> MGDSILSQAEIDA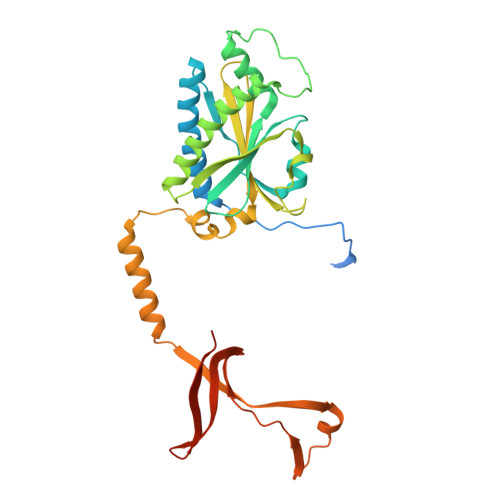LLNGDSDTKDEPTPGIASDSDIRPYDPNTQRRVVRERLQALEIINERFARQFRMGLFNLLRRSPDITVGAIRIQPYHEFARNLPVPTNLNLIHLKPLRGTGLVVFSPSLVFIAVDNLFGGDGRFPTKVEGREFTHTEQRVINRMLKLALEGYSDAWKAINPLEVEYVRSEMQVKFTNITTSPNDIVVNTPFHVEIGNLTGEFNICLPFSMIEPLRELLVNPPLENSRHEDQNWRDNLVRQVQHSELELVANFADIPLRLSQILKLKPGDVLPIEKPDRIIAHVDGVPVLTSQYGTVNGQYALRVEHLINPILNSLNEEQPK> MQSSALRPSSLLRAYHYVHPKTGRPIRQYRKYGDPRFINNEVALIKGLFALITTDFGMVTQSQLENARLAILRRMPRGSFALTMHTDYEEFPVVQKSPESRMGAGKSNIHHFAYKFTTGVPLFEITALSSRRLNQAEAEGI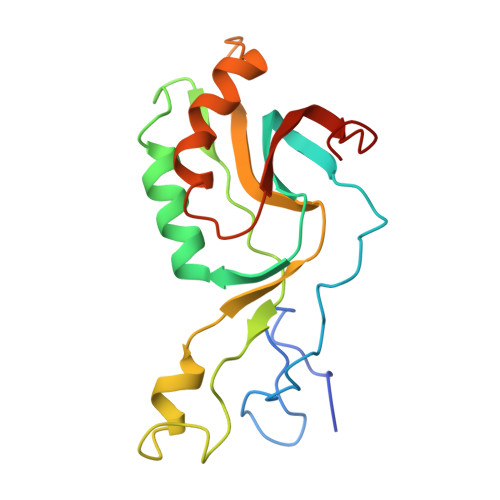FLAGRSFIPLQTAVVPRGRVDEYHVFK> MDEADRRLLRRCRLRLVEELQVDQLWDALLSRELFRPH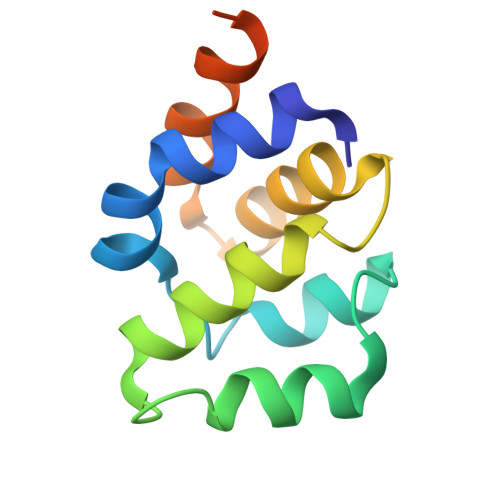MIEDIQRAGSGSRRDQARQLIIDLETRGSQALPLFISCLEDTGQDMLASFLRTNRQAAKLSKLEHHHHHH>GGGSMEVVGDFEYSKRDLVGHGAFAVVFRGRHRQKTDWEVAIKSINKKNLSKSQILLGKEIKILKELQHENIVALYDVQELPNSVFLVMEYCNGGDLADYLQAKGTLSEDTIRVFLHQIAAAMRILHSKGIIHRDLKPQNILLSYANRRKSSVSGIRIKIADFGFARYLHSNMMAADLCGSPMYMAPEVIMSQHYDAKADLWSIGTVIYQCLVGKPPFQANSPQDLRMFYEKNRSLMPSIPRETSPYLANLLL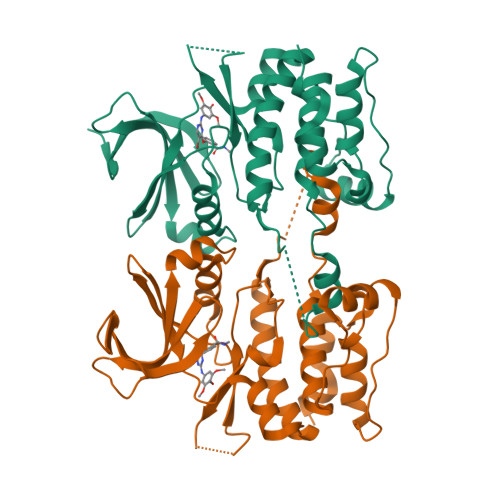GLLQRNQKDRMDFEAFFSHPFLEQGPV[4x]> GPEFLSNKQTHWYYFKLPGLNSRQWKGPQEALQEAAGAALIPVSASSAQWIPWRLLKRAACPRPVGGPA

IN first catalyses 3′-processing of the vDNA ends, exposing reactive 3′ OH nucleophile groups that it uses to attack a pair of phosphodiester bonds within target DNA (tDNA), resulting in strand transfer. In this work, we determine the three-dimensional structure of the deltaretroviral intasome and characterize its interactions with its host factor, the PP2A-B56γ subunit. The deltaretroviral IN host cofactor B56γ14, as part of the heterotrimeric protein phosphatase 2A (PP2A) holoenzyme, interacts with a number of chromatin-associated proteins and potently stimulates concerted integration activity of deltaretroviral INs14.

To aid the interpretation of the cryo-EM map, we generated a high-quality homology model of the STLV-1 IN/NTD using the SWISS-MODEL server, and determined a series of X-ray crystal structures spanning the catalytic core domain (CCD) and the C-terminal domain (CTD) of HTLV-2 and -1 IN. The IN/CTD structure was determined in isolation as well as in complex with B56γ. While the canonical IN/CCD dimer observed in crystals could be docked directly into the cryo-EM map, the CTDs could only be docked as monomers. We speculate that the dimers and trimers observed in IN/CTD crystals may be relevant within viral particles prior to vDNA synthesis by reverse transcription.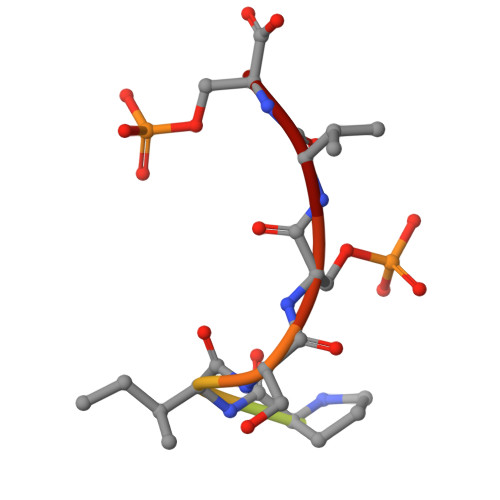> SPHNPISSVS>MHSGIDIRVARPEDAEEIQIIYAPIVLNTAISFEEAVPSVEQMRERISTTLQTYPYLVAVREGRVVGYAYASQHRARAAYRWAVDVTVYVAEGQRRSGIARQLYDVLLPVLKRLGYRSAYAGIALPNEGSVGLHERLGFQHIGTFPQVGFKLDAWHDVGYWRFDFGDEGLHPEAPLGFLSQIPLGPEQKLISEEDLNSAVDHHHHHH[2x]

The arsN1 gene encodes an N-acetyltransferase that confers resistance to arsinothricin with high selectivity over the related antibiotic phosphinothricin. Here we show that ArsN1 acetylates both AST and PPT but with higher affinity for AST, indicating that ArsN1 is an AST-selective N-acetyltransferase. The overall conformation is a three-layer α/β sandwich fold, a typical GCN5-related N-acetyltransferase fold. PpArsN1 forms an asymmetric homodimer in solution, as shown by the extensive interactions of the subunits and size-exclusion chromatography, similar to related N-acetyltransferases.

To elucidate the mechanism of PpArsN1 resistance and its selectivity for AST, we solved the structure of apo- and substrate-bound PpArsN1. Arg75a in Chain A of the apo-structure also shows two conformations. One superimposes with the L-AST-bound PpArsN1 structure, covering the substrate-binding channel, whereas the other moves out of channel. The side chain of Arg77b in Chain B also appears to cover and move away from the substrate-binding site, allowing substrate access to the active site. The two conformations of this residue in L-PPT-bound PpArsN1, for both PPT-1 and PPT-2, are quite similar to those in L-AST-bound PpArsN1. Arg75 and Arg77 from each subunit appear to form gates that controls substrate access to both catalytic sites.>MYRK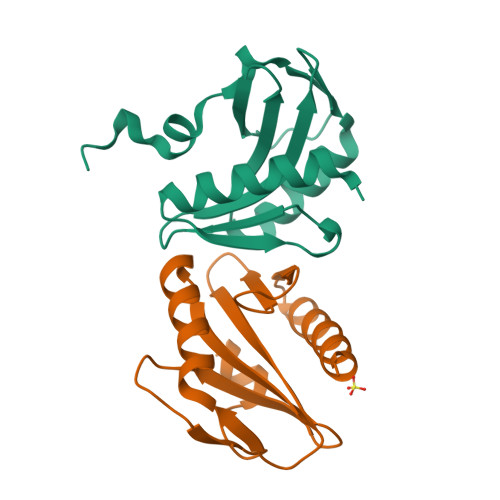GAQAERELIKLLEKHGFAVVRSAGSKKVDLVAGNGKKYLCIEVKVTKKDHLYVGKRDMGRLIEFSRRFGGIPVLAVKFLNVGWRFIEVSPKIEKFVFTPSSGVSLEVLLGIQKTLEGKS[4x]>MILMRRTLKAAILGATGLVGIEYVRMLSNHPYIKPAYLAGKGSVGKPYGEVVRWQTVGQVPKEIADMEIKPTDPKLMDDVDIIFSPLPQGAAGPVEEQFAKEGFPVISNSPDHRFDPD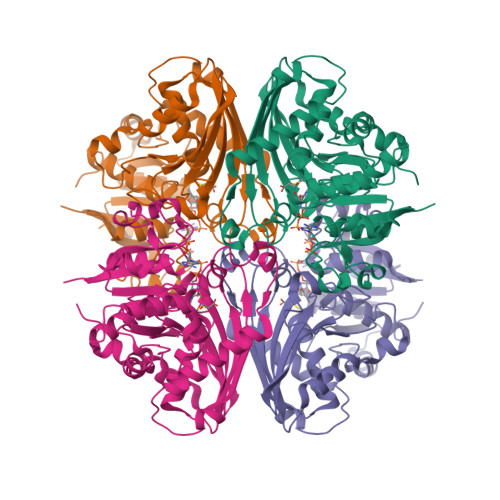VPLLVPELNPHTISLIDEQRKRREWKGFIVTTPLCTAQGAAIPLGAIFKDYKMDGAFITTIQSLSGAGYPGIPSLDVVDNILPLGDGYDAKTIKEIFRILSEVKRNVDEPKLEDVSLAATTHRIATIHGHYEVLYVSFKEETAAEKVKETLENFRGEPQDLKLPTAPSKPIIVMNEDTRPQVYFDRWAGDIPGMSVVVGRLKQVNKRMIRLVSLIHNTVRGAAGGGILAAELLVEKGYIEK[4x]> MSTLCPPPSPAVAKTEIALSGKSPLLAATFAYWDNILGPRVRHIWAPKTEQVLLSDGEITFLANHTLNGEILRNAESGAIDVKFFVLSEKGVIIVSLIFDGNWNGDRSTYGLSIILPQTELSFYLPLHRVCVDRLTHIIRKGRIWMHKERQENVQKIILEGTERMEDQGQSIIPMLTGEVIPVMELLSSMKSHSVPEEIDIADTVLNDDDIGDSCHEGFLLNAISSHLQTCGCSVVVGSSAEKVNKIVRTLCLFLTPAERKCSRLCEAESSFKYESGLFVQGLLKDSTGSFVLPFRQVMYAPYPTTHIDVDVNTVKQMPPCHEHIYNQRRYMRSELTAFWRATSEEDMAQDTIIYTDESFTPDLNIFQDVLHRDTL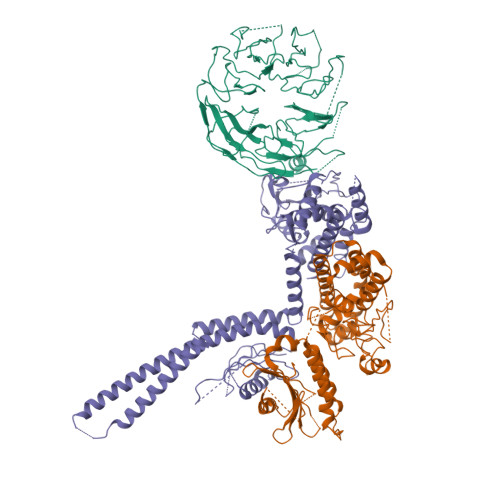VKAFLDQVFQLKPGLSLRSTFLAQFLLVLHRKALTLIKYIEDDTQKGKKPFKSLRNLKIDLDLTAEGDLNIIMALAEKIKPGLHSFIFGRPFYTSVQERDVLMTF;> MISAPDVVAFTKEEEYEEEPYNEPALPEEYSVPLFPFASQGANPWSKLSGAKFSRDFILISEFSEQVGPQPLLTIPNDTKVFGTFDLNYFSLRIMSVDYQASFVGHPPGSAYPKLNFVEDSKVVLGDSKEGAFAYVHHLTLYDLEARGFVRPFCMAYISADQHKIMQQFQELSAEFSRASECLKTGNRKAFAGELEKKLKDLDYTRTVLHTETEIQKKANDKGFYSSQAIEKANELASVEKSIIEHQDLLKQIRSYPHRKLKGHDLCPGEMEHIQDQASQASTTSNPDESADTDLYTCRPAYTPKLIKAKSTKCFDKKLKTLEELCDTEYFTQTLAQLSHIEHMFRGDLCYLLTSQIDRALLKQQHITNFLFEDFVEVDDRMVEKQESIPSKPSQDRPPSSSLEECPIPKVLISVGSYKSSVESVLIKMEQELGDEEYKEVEVTELSSFDPQENLDYLDMDMKGSISSGESIEVLGTEKSTSVLSKSDSQASLTVPLSPQVVRSKAVSHRTISEDSIEVLSTCPSEALIPDDFKASYPSAINEEESYPDGNEGAIRFQASISPPELGETEEGSIENTPSQIDSSCCIGKESDGQLVLPSTPAHTHSDEDGVVSSPPQRHRQKDQGFRVDFSVENANPSSRDNSCEGFPAYELDPSHLLASRDISKTSLDNYSDTTSYVSSVASTSSDRIPSAYPAGLSSDRHKKRAGQNALKFIRQYPFAHPAIYSLLSGRTLVVLGEDEAIVRKLVTALAIFVPSYGCYAKPVKHWASSPLHIMDFQKWKLIGLQRVASPAGAGTLHALSRYSRYTSILDLDNKTLRCPLYRGTLVPRLADHRTQIKRGSTYYLHVQSMLTQLCSKAFLYTFCHHLHLPTHDKETEELVASRQMSFLKLTLGLVNEDVRVVQYLAELLKLHYMQESPGTSHPMLRFDYVPSFLYKI;> MLRWLIGGGREPQGLAEKSPLQTIGEEQTQNPYTELLVLKAHHDIVRFLVQLDDYRFASAGDDGIVVVWNAQTGEKLLELNGHTQKITAIITFPSLESCEEKNQLILTASADRTVIVWDGDTTRQVQRISCFQSTVKCLTVLQRLDVWLSGGNDLCVWNRKLDLLCKTSHLSDTGISALVEIPKNCVVAAVGKELIIFRLVAPTEGSLEWDILEVKRLLDHQDNILSLINVNDLSFVTGSHVGELIIWDALDWTMQAYERNFWDPSPQLDTQQEIKLCQKSNDISIHHFTCDEENVFAAVGRGLYVYSLQMKRVIACQKTAHDSNVLHVARLPNRQLISCSEDGSVRIWELREKQQLAAEPVPTGFFNMWGFGRVSKQASQPVKKQQENATSCSLELIGDLIGHSSSVEMFLYFEDHGLVTCSADHLIILWKNGERESGLRSLRLFQKLEENGDLYLAV> HGSPVDICTAKPRDIPMNPMCIYRSPEKKATEDEGSEQKIPEATNRRVWELSKANSRFATTFYQHLADSKNDNDNIFLSPLSISTAFAMTKLGACNDTLQQLMEVFKFDTISEKTSDQIHFFFAKLNCRLYRKANKASKLVSANRLFGDKSLTFNETYQDISELVYGAKLQPLDFKENAEQSRAAINKWVSNKTEGRITDVIPSEAINELTVLVLVNTIYFKGLWKSKFSPENTRKELFYKADGESCSASMMYQEGKFRYRRVAEGTQVLELPFKGDDITMVLILPKPEKSLAKVEKELTPEVLQEWLDELEEMMLVVHMPRFRIEDGFSLKEQLQDMGLVDLFSPEKSKLPGIVAEGRDDLYVSDAFHKAFLEVNEEGSEAAAS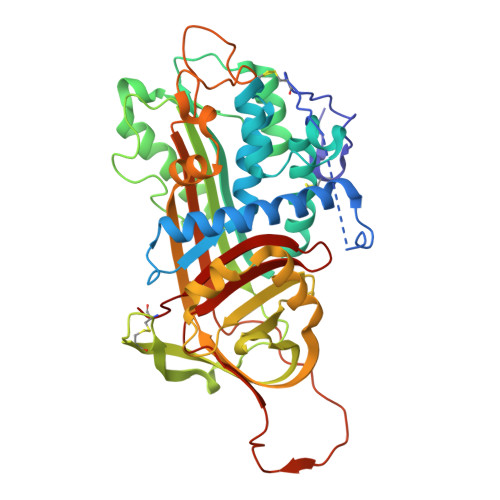TAVVIAGRSLNPNRVTFKANRPFLVFIREVPLNTIIFMGRVANPCVK>MGSLVNRKQLEKMANVRFRTQEDEYVAILDALEEYHNMSENTVVEKYLKLKDINSLTDIYIDTYKKSGRNKALKKFKEYLVTEVLELKNNNLTPVEKNLHFVWIGGQINDTAINYINQWKDVNSDYNVNVFYDSNAFLINTLKKTVVESAINDTLESFRENLNDPRFDYNKFFRKRMEIIYDKQKNFINYYKAQREENPELIIDDIVKTYLSNEYSKEIDELNTYIEESLNKITQNSGNDVRNFEEFKNGESFNLYEQELVERWNLAAASDILRISALKEIGGMYLDVDMLPGIQPDLFESIEKPSSVTVDFWEMTKLEAIMKYKEYIPEYTSEHFDMLDEEVQSSFESVLASKSDKSEIFSSLGDMEASPLEVKIAFNSKGIINQGLISVKDSYCSNLIVKQIENRYKILNNSLNPAISEDNDFNTTTNTFIDSIMAEANADNGRFMMELGKYLRVGFFPDVKTTINLSGPEAYAAAYQDLLMFKEGSMNIHLIEADLRNFEISKTNISQSTEQEMASLWSFDDARAKAQFEEYKRNYFEGSLLEHHHHHH[2x]

TcdA and TcdB bacterial toxins are primary determinants of disease pathogenesis and are attractive therapeutic targets. TcdA and TcdB contain domains that use UDP-glucose to glucosylate and inactivate host Rho GTPases, resulting in cytoskeletal changes causing cell rounding and loss of intestinal integrity. The GTD domains of TcdA and TcdB catalyze transfer of a glucosyl residue to a nucleophilic threonine acceptor in Rho GTPases. Iminosugars, isofagomine and noeuromycin mimic the transition state and inhibit both TcdA and TcdB by forming ternary complexes with Tcd and UDP, a product of the TcdA- and TcdB-catalyzed reactions.

The geometry of UDP, isofagomine and noeuromycin bound to TcdB-GTD was established by solving the crystal structures. The binding of UDP and isofagomine is well resolved in the binding pocket. The uracil ring is π-π stacked with Trp102 and sandwiched between the side chains of Trp102 and Leu265. The α and β phosphates of UDP also interact with structural waters and coordinate to the Mn2+ metal cation, which is in turn coordinated to the carboxyl groups of Asp288 and Glu515. The cationic nitrogen of isofagomine is 2.6 Å from O of the β-phosphate of UDP in an ion-pair interaction. A structural water molecule is 2.7 Å on the opposite face of the isofagomine cation in appropriate position to act as the attacking nucleophile for the hydrolytic reaction of TcdB with UDP-glucose. O3 of isofagomine is hydrogen bonded with the carboxylate of Asp286 and the Arg273 guanidinium. The O4 and O6 of the isofagomine share H-bond interactions with both carboxylate oxygens of Asp270. Movement of the loop from residues Gln510 to Asp523 (10 Å) towards the binding pocket occurs on inhibitor binding and is highlighted with the black arrow. The entropic contribution for isofagomine and noeuromycin binding was –TΔS = 0.5 ± 0.2 kcal/mol and -TΔS = 4.2 ± 0.3 kcal/mol, respectively. Larger enthalpic contributions of isofagomine binding to TcdB-GTD in the presence of UDP is consistent with the Ki values presented in Table 2, making isofagomine the more potent inhibitor.> MGHHHHHHHHHHSSGMTELPPNAPNPENATNELAQELLRKLRQKQGNWVEWGQAIASLQKSGYNPQDIFEATGFEPVQQNQVIVGSQVYNSLEKSGASAATLAHYATRGSDVLYELRLLTHEERAAAGDLTFTHKVDADEAREIAKAIKDFSRFRILPEGFSNHPGDAVAYQAWKLA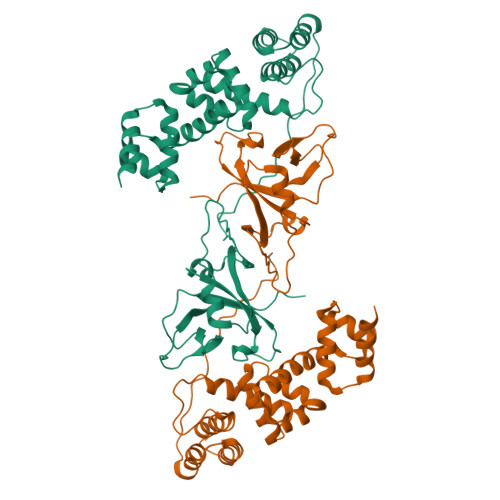RQYSDLQERSRLIARGLRFAHSETARKQIEQLLVDFTVVSQRPAPIPPFFRFDTEDELPRIVPVVGQLPLKAEELKAVPLVEEIEPFRLVKFSGEQAWVALPGWQVLLAAEDPVTILATSDRFPKQNQTEPGPVLVVVDRSQREWNDFSYFVVDHDGELDFQWFETKPEFPILGKVIILVRPRRILDENVTKDSWQIDE>GSHMGEIRPTIGQQMETGDQRFGDLVFRQLAPNVWQHTSYLDMPGFGAVASNGLIVRDGGRVLVVDTAWTDDQTAQILNWIKQEINLPVALAVVTHAHQDKMGGMDALHAAGIATYANALSNQLAPQEGMVAAQHSLTFAANGWVEPATAPNFGPLKVFYPGPGHTSDNITVGIDGTDIAFGGCLIKDSKAKS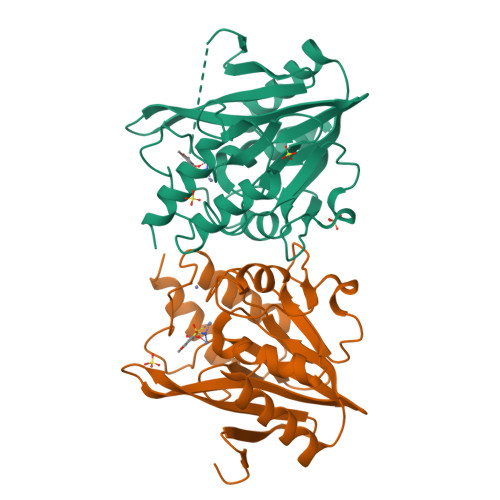LGNLGDADTEHYAASARAFGAAFPKASMIVMSHSAPDSRAAITHTARMADKLR[2x]> MGRILFLTTFMSKGNKVVRYLESLHHEVVICQEKVHAQSANLQEIDWIVSYAYGYILDKEIVSRFRGRIINLHPSLLPWNKGRDPVFWSVWDETPKGVTIHLIDEHVDTGDILVQEEIAFADEDTLLDCYNKANQAIEELFIREWENIVHGRIAPYRQTAGGTLHFKADRDFYKNLNMTTVRELLALKRLCAEPKRGEKPIDKTFHQLFEQQVEMTPDHVAVVDRGQSLTYKQLNERANQLAHHLRGKGVKPDDQVAIMLDKSLDMIVSILAVMKAGGAYVPIDPDYPGERIAYMLADSSAAILLTNALHEEKANGACDIIDVHDPDSYSENTNNLPHVNRPDDLVYVMYTSGSTGLAKGVMIEHHNLVNFCEWYRPYFGVTPADKALVYSSFSFDGSALDIFTHLLAGAALHIVPSERKYDLDALNDYCNQEGITISYLPTGAAEQFMQMDNQSFRVVITGGDVLKKIERNGTYKLYNGYGPTECTIMVTMFEVDKPYANIPIGKPIDRTRILILDEALALQPIGVAGELFIVGEGLGRGYLNRPELTAEKFIVHPQTGERMYRTGDRARFLPDGNIEFLGRLDNLVKIRGYRIEPGEIEPFLMNHPLIELTTVLAKEQA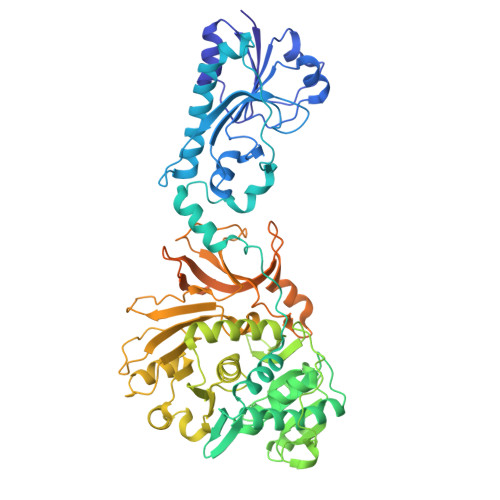DGRKYLVGYYVAPEEIPHGELREWLGNDLPDYMIPTYFVHMKAFPLTANGKVDRRALPDVQADA> PPENFLEI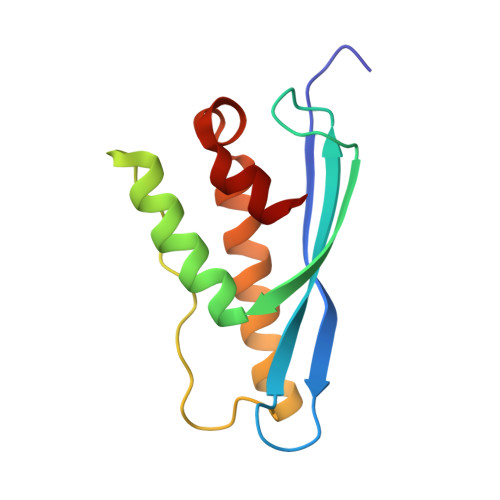EVRNPQTHGVGRHMYTDYEIVCRTNIPAFKLRQSSVRRRYSDFEYFRDILERESARVTIPPLPGKVFTNRFSDEVIENRRAGLEKFLKIVVGHPLLQTGSKVLAAFVQ(2~{R},3~{S},4~{S},5~{R},6~{S})-2-(hydroxymethyl)-6-[(2~{R},3~{R},4~{S},5~{R},6~{S})-2-(hydroxymethyl)-6-[(2~{R},3~{R},4~{S},5~{R},6~{R})-2-(hydroxymethyl)-3,5-bis(oxidanyl)-6-[4-(3-pyridin-1-ium-1-ylpropyl)-1,2,3-triazol-1-yl]oxan-4-yl]oxy-3,5-bis(oxidanyl)oxan-4-yl]oxy-oxane-3,4,5-triol 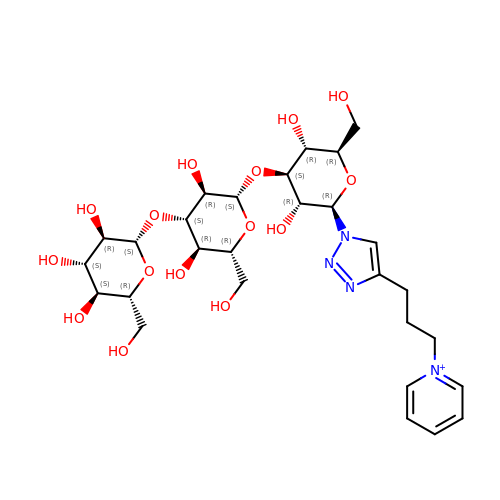| C28 H43 N4 O15 | KBNJHYMTJQZFJJ-ZJLPYKFYSA-N2′,3′-cyclic nucleotide 3′-phosphodiesterase (CNPase) comprises 4% of total myelin protein in the central nervous system (CNS), being the most abundant CNS non-compact myelin protein4. CNPase consists of an N-terminal polynucleotide kinase-like domain10, a catalytic phosphodiesterase domain11, and a membrane-anchored C-terminal tail, which contains a cysteine residue that undergoes isoprenylation. The catalytic domain enables the rapid hydrolysis of nucleoside 2′,3′-cyclic phosphates to nucleoside 2′-phosphates. The CNPase catalytic site, lying in a groove between two lobes, has pseudo two-fold symmetry and contains two apposing His-X-Thr-X (X denotes a hydrophobic residue) motifs, characteristic for 2H phosphoesterases 113537.

In mouse CNPase, this is done by His230, Thr232, His309, and Thr311, in a manner, where a nucleophilic water molecule activated by His309 can attack the cyclic phosphate and a pentavalent transition state is formed. Mutation of active-site histidine residues (H230Q, H230S, H309Q, H309S, and H230Q/H309Q double mutant) abolishes CNPase activity. Overall, the structures of H230S, H309S, H230Q, H309Q, and H230Q/H309Q are highly similar. However, only H230S and H309S could be used to trap nucleotide ligands within the active site, whereas H309Q and the H230Q/H309Q double mutant could not.

> GGLEKDFLPLYFGWFLTKKSSETLRKAGQVFLEELGNHKAFKKELRHFISGDEPKEKLELVSYFGKRPPGVLHCTTKFCDYGKAAGAEEYAQQEVVKRSYGKAFKLSISALFVTPKTAGAQVVLTDQELQLWPSDLDKPSASEGLPPGSRAQVTLGCAADVQPVQTGLDLLDILQQVKGGSQGEAVGELPRGKLYSLGKGRWMLSLTKKMEVKAIFTGYYG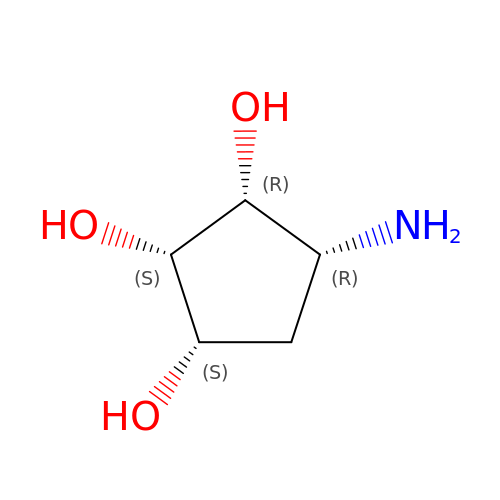(1S,2S,3R,4R)-4-aminocyclopentane-1,2,3-triol | C5 H11 N O3 | UUKWSEIZIMUXPU-LECHCGJUSA-N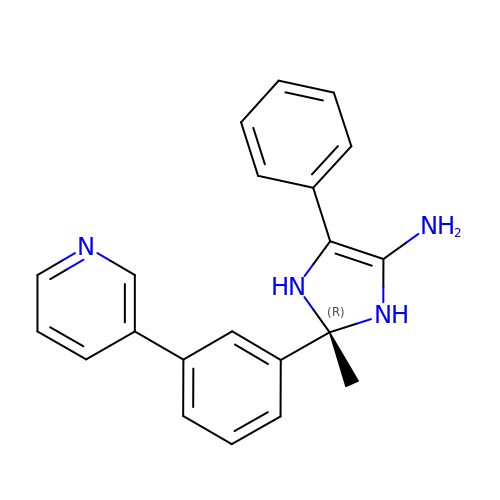(2R)-2-methyl-5-phenyl-2-(3-pyridin-3-ylphenyl)-2,3-dihydro-1H-imidazol-4-amine | C21 H20 N4 | BLSGQDNQCUBPGO-OAQYLSRUSA-N> MGSSHHHHHHSSGLVPRGSMSTSWSDRLQNAADMPANMDKHALKKYRREAYHRVFVNRSLAMEKIKCFGFDMDYTLAVYKSPEYESLGFELTVERLVSIGYPQELLSFAYDSTFPTRGLVFDTLYGNLLKVDAYGNLLVCAHGFNFIRGPETREQYPNKFIQRDDTERFYILNTLFNLPETYLLACLVDFFTNCPRYTSCETGFKDGDLFMSYRSMFQDVRDAVDWVHYKGSLKEKTVENLEKYVVKDGKLPLLLSRMKEVGKVFLATNSDYKYTDKIMTYLFDFPHGPKPGSSHRPWQSYFDLILVDARKPLFFGEGTVLRQVDTKTGKLKIGTYTGPLQHGIVYSGGSSDTICDLLGAKGKDILYIGDHIFGDILKSKKRQGWRTFLVIPE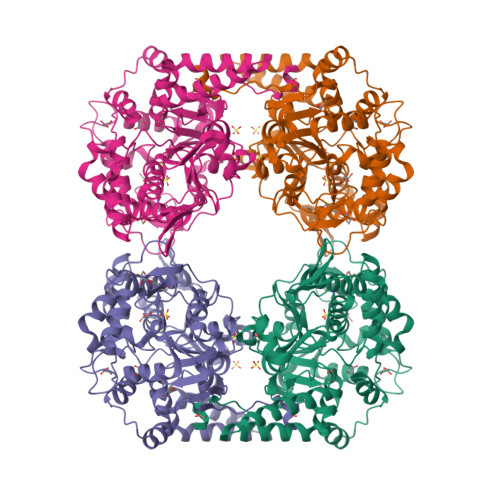LAQELHVWTDKSSLFEELQSLDIFLAELYKHLDSSSNERPDISSIQRRIKKVTHDMDMCYGMMGSLFRSGSRQTLFASQVMRYADLYAASFINLLYYPFSYLFRAAHVLMPHESTVEHTHVDINEMESPLATRNRTSVDFKDTDYKRHQLTRSISEIKPPNL>[3x]MENSKTEQVTGATGITQSTVTAPLPEAVSSLSLAPTVNALDPWVYLNQTEVPGGTFTVSSATQPGSVLLELEISPELNLYTSHLFRMYAGWSGGFSLKLLVAGNAFSAGKLIAAIIPPNIEVPNSAYLLTGFPHEILDFRTADSMEIIAPDIKNIDYHFRGDKLGKLVVMVYSPLRSTSADFEIEIKLTSAPLPDFKFTMLVPPIQNNALPIWSIPQAPPYSMVNPRSPLTPVVELYINSSYATCNHQLGRYTIYQGAIGNSTFNPSGAWTATCTAEAGSVTGNPNWRYALLDLPDNPTFDPTLPPVPRGFCDWGSGVKSGNKQHLVCFTGKKFAGGFQDVDAHMWDYGDNETVGLDNTYQRTIYISDPSLEKDAQYLVIPMGVSGAANDDTVQVAPNCYGSWDYAPTVAPPLGEQFVWFRSQLPASKTTTTSGVNSVPVNVNALMSPDLIRSAYASGFPLGKVALLDYVLFGGSVVRQFKLYPEGYMTANTTGSNTGFIIPADGYFRFNSWVSPSFMISSVVDLNLQTAVVFR

Caliciviruses are a diverse group of non-enveloped, positive-sense RNA viruses with a wide range of hosts and transmission routes. One area of calicivirus biology that has gained increasing attention over the past decade is the conformational flexibility exhibited by the protruding (P) domains of the major capsid protein VP1. This was observed in structure analyses of capsids encoded by many species and is often a consequence of environmental cues such as metal ions, changes to pH, or receptor/co-factor engagement. The ability of P-domains to undergo conformational shifts according to environmental conditions plays a crucial role in infection, significantly influencing both receptor binding and entry, and enabling evasion of the host immune response.

Although recently, organoid and in vivo models for HuNoV infection have been reported, these studies are still in their infancy and most of our current understanding of HuNoV has been inferred from other cultivatable members of the Caliciviridae, such as murine norovirus (MNV), FCV, and Tulane virus (TuV). These viruses have been widely used in structural, infectivity, environmental survivability, and disinfection studies due to their genetic and structural similarities to HuNoV. We provide new data to show that conformational flexibility in TuV capsids, for which we have yet to identify an environmental cue, varies between preparations, potentially frustrating efforts to study entry. In TuV and RHDV, this increased flexibility appeared to be caused by significantly reduced interactions between the shell and P1-domain in C/C dimers, compared to A/B dimers. While the purpose of this is unknown, it was suggested that this particularly flexible state could facilitate interactions with host cell co-factors. Nevertheless, the effects of different conformational dynamics between A/B and C/C dimers should be taken into account when considering calicivirus interactions with receptors and cofactors. While it can be assumed that the mechanism and purpose of P-domain movement is well-conserved among the Caliciviridae, it is still important to characterise P-domain conformational dynamics in other HuNoV surrogates, such as TuV and porcine sapovirus, as well as enteric strains of FCV.> TFAYKIDGNEVIFTLWAPYQKSVKLKVLEKGLYEMERDEKGYFTITLNNVKVRDRYKYVLDDASEIPDPASRYQPEGVHGPSQIIQESKEFNNETFLKK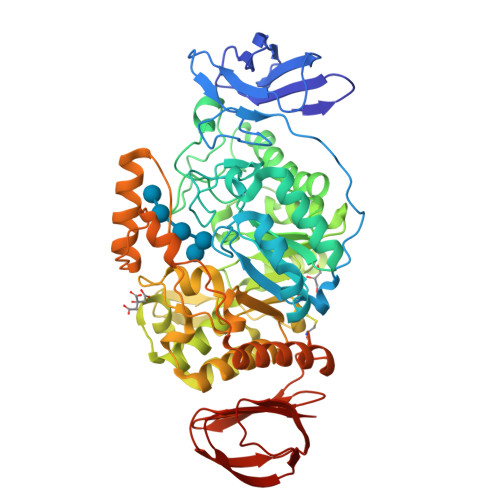EDLIIYEIHVGTFTPEGTFEGVIRKLDYLKDLGITAIEIMPIAQFPGKRDWGYDGVYLYAVQNSYGGPEGFRKLVDEAHKKGLGVILDVVYNHVGPEGNYMVKLGPYFSQKYKTPWGLTFNFDDAESDEVRKFILENVEYWIKEYNVDGFRLDAVHAIIDTSPKHILEEIADVVHKYNRIVIAQSDLNDPRVVNPKEKCGYNIDAQWVDDFHHSIHAYLTGERQGYYTDFGNLDDIVKSYKDVFVYDGKYSNFRRKTHGEPVGELDGCNFVVYIQNHDQVGNRGKGERIIKLVDRESYKIAAALYLLSPYIPMIFMGEEYGEENPFYFFSDFSDSKLIQGVREGRKKENGQDTDPQDESTFNASKLSWKIDEEIFSFYKILIKMRKELSIACDRRVNVVNGENWLIIKGREYFSLYVFSKSSIEVKYSGTLLLSSNNSFPQHIEEGKYEFDKGFALYKL2-AMINO-9-(2-DEOXY-3-O-PHOSPHONOPENTOFURANOSYL)-1,9-DIHYDRO-6H-PURIN-6-ONE | C10 H14 N5 O7 P | 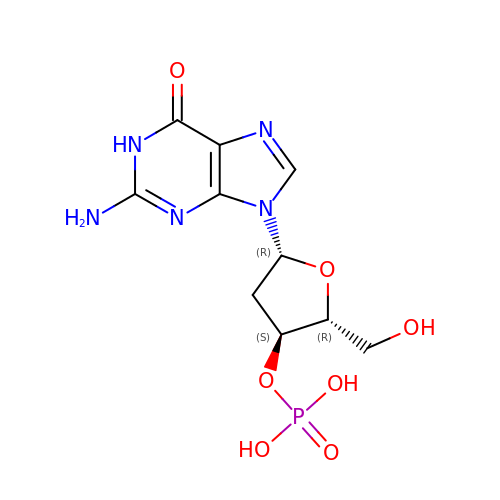QQMSZHORHNORLP-KVQBGUIXSA-N>[6x]GGDLANEIARCTKLLNALNSGGDLANEIARCTKLLNALNSGGDLANE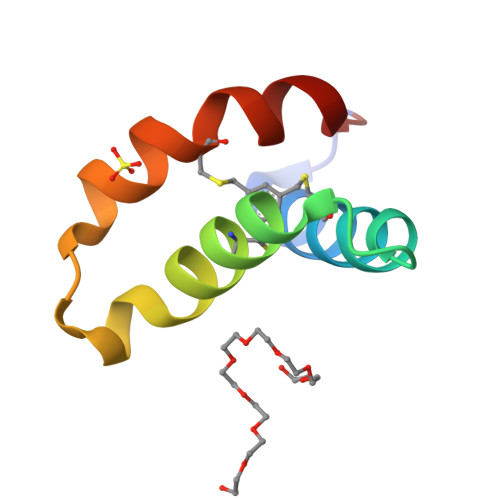IARCTKLLNALNS(1R,3AS,4R,8AS,8BR)-4-(2-BENZO[1,3]DIOXOL-5-YLMETHYL-1-ISOPROPYL-3-OXO-DECAHYDRO-PYRROLO[3,4-A]PYRROLIZIN-4-YL)-BENZAMIDINE 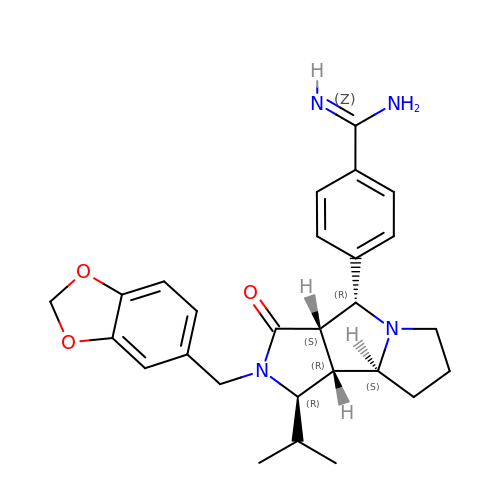| C27 H32 N4 O3 | TZROHICTGLJYJF-FTSNLURZSA-N>MGSSHHHHHHSQDPKPLKTYVDPHTYEDPNQAVLKFTTEIHPSCVTRQKVIGAGEFGEVYKGMLKTSSGKKEVPVAI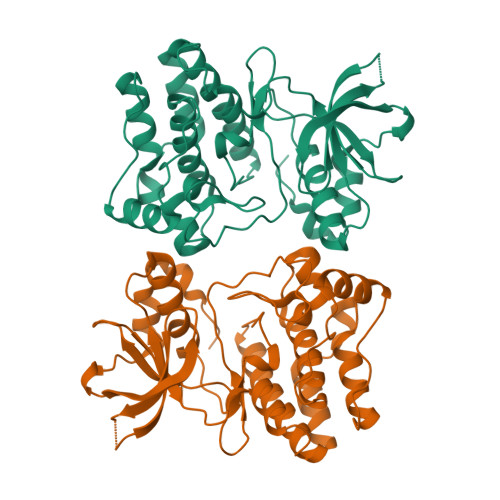KTLKAGYTEKQRVDFLGEAGIMGQFSHHNIIRLEGVISKYKPMMIITEYMENGALDKFLREKDGEFSVLQLVGMLRGIAAGMKYLANMNYVHRDLAARNILVNSNLVCKVSDFGLSRVLEDDPEATYTTSGGKIPIRWTAPEAISYRKFTSASDVWSFGIVMWEVMTYGERPYWELSNHEVMKAINDGFRLPTPMDCPSAIYQLMMQCWQQERARRPKFADIVSILDKLIR[2x]3-{[(2S)-2-amino-2-carboxyethyl]sulfanyl}-5-hydroxy-L-tyrosine | C12 H16 N2 O6 S | 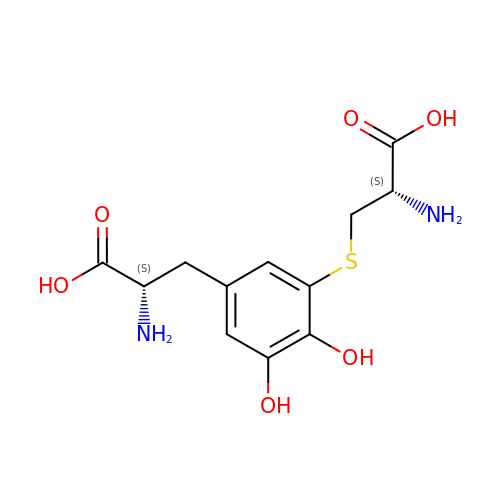SXISMOAILJWTID-NKWVEPMBSA-N>MKKIITLFGACALAFSMANADVNLYGPG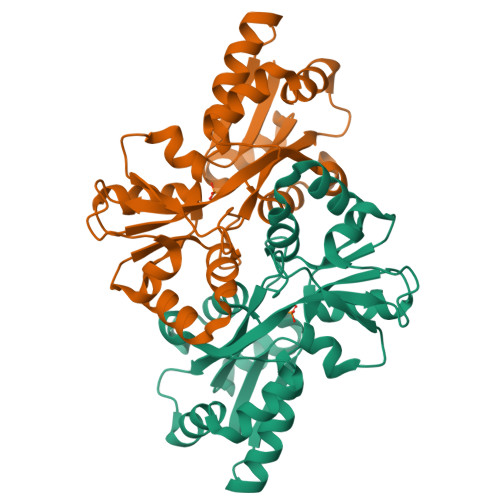GPHTALKDIANKYSEKTGVKVNVNFGPQATWFEKAKKDADILFGASDQSALAIASDFGKDFNVSKIKPLYFREAIILTQKGNPLKIKGLKDLANKKVRIVVPEGAGKSNTSGTGVWEDMIGRTQDIKTIQNFRNNIVAFVPNSGSARKLFAQDQADAWITWIDWSKSNPDIGTAVAIEKDLVVYRTFNVIAKEGASKETQDFIAYLSSKEAKEIFKKYGWREH[2x]>GSHMAHAMENSWTISKEYHIDEEVGFALPNPQENLPDFYNDWMFIAKHLPDLIESGQLRERVEKLNMLSIDHLTDHKSQRLARLVLGCITMAYVWGKGHGDVRKVLPRNIAVPYCQLSKKLELPPILVYADCVLANWKKKDPNKPLTYENMDVLFSFRDGDCSKGFFLVSLLVEIAAASAIKVIPTVFKAMQMQERDTLLKALLEIASCLEKALQVFHQIHDHVNPKAFFSVLRIYLSGWKGNPQLSDGLVYEGFWEDPKEFAGGSAGQSSVFQCFDVLLGIQQTAGGG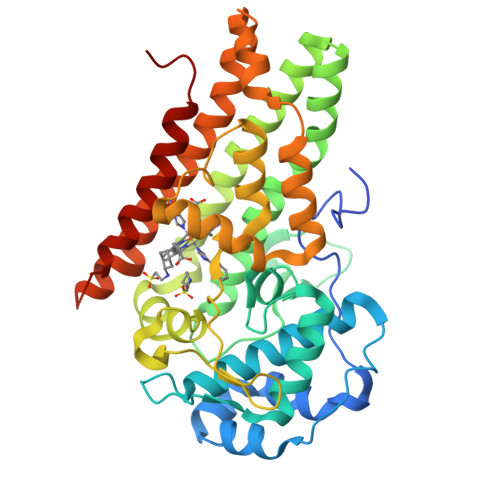HAAQFLQDMRRYMPPAHRNFLCSLESNPSVREFVLSKGDAGLREAYDACVKALVSLRSYHLQIVTKYILIPASQQPKENKTSEDPSKLEAKGTGGTDLMNFLKTVRSTTEKSLLKEG[2x]> KSTVEKSTVGQKVAIVREDTGTIAELAEKALGNMVDIVYAGSDLKEAEEAVKKEKAPAIIVIPKGFSQSLESGEKARLEIVWYLRGTGLSEA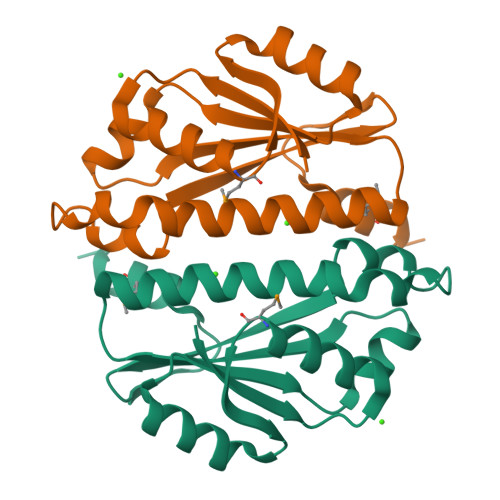VSTGTISSLIESLKVQLASFLLNDPKKAQLLFDPLEIVQHTYLRGSLFKNHSPEAIMNVFYSQN> MGKSHSPVHWKSAAEIVELVKSKQISPREVVESTIDLIEQRDPGLNAVVYKAYDEARE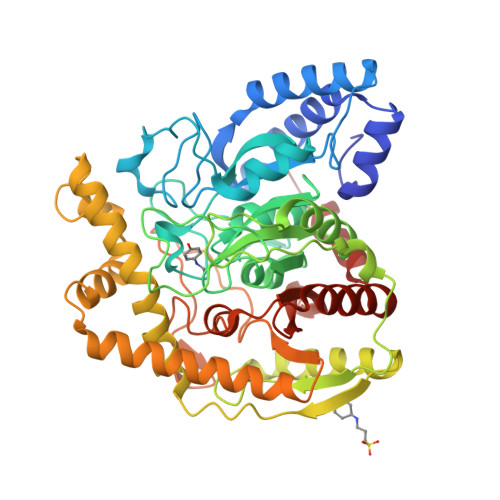KAAALERRIMQGEPVGMLAGVPTLMKDLFAAKPGWPSTLGGIRALKDARGAAGVWSTYPLKMSGEDSLLLGQTNSPVYGFRGTTDNTFFGPTRNPFNLDFNAGGSSGGAAALVADGIVPVAGGTDGGGAIRIPAAWTNTYGFQPSIGRVPFKSRPNAFHPGPYLYEGPITRTVRDAALAMNVLHGFDRRDPASLRVKLDFTSALAQGVRGKKIGLTLNYGVFPVQQEIQDLIGKAARVFTELGAHVEFVDLGIPYSQKQMSDAWCRMIAIPTVASMQALRKEGIDLYGEHRADIPDALMKWIDAVADISVQQISADQLLRTTVFDCMNGVFDRFDLLLAPTLACMPVRNATDGCTEGPSQINGEEIDPLIGWCMTYLTNFSGHPSASVPAGLIDGLPAGMLIIGDRQADLDVIAASAAFERASPWSQYYDIPAGRPL>SVKLAGNSSLCPVSGWAIYSKDNSVRIGSKGDVFVIREPFISCSPLECRTFFLTQGALLNDKHSNGTIKDRSPYRTLMSCPIGEVPSPYNSRFESVAWSASACHDGINWLTIGISGPDNGAVAVLKYNGIITDTIKSWRNNILRTQESECACVNGSCFTVMTDGPSNGQASYKIFRIEKGKIVKSVEMNAPNYHYEECSCYPDSSEITCVCRDNWHGSNRPWVSFNQNLEYQIGYICSGIFGDNPRPNDKTGSCGPVSSNGANGVKGFSFKYGNGVWIGRTKSISSRNGFEMIWDPNGWTGTDNNFSIKQDIVGINEWSGYSGSFVQHPELTG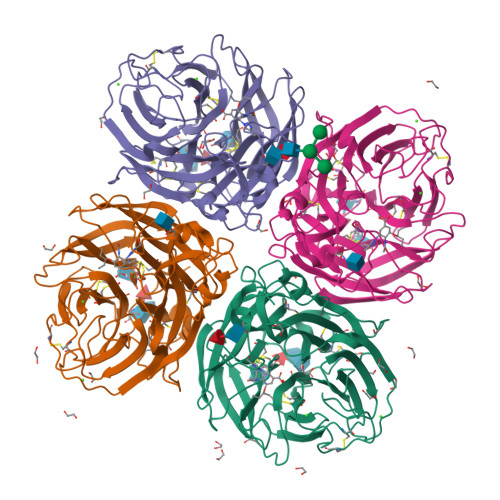LDCIRPCFWVELIRGRPKENTIWTSGSSISFCGVNSDTVGWSWPDGAELPFTIDK[4x]>LFIEWL[4x]

Here, we identify an evolutionarily conserved hexapeptide sequence as the major aggregation-prone region (APR) of gastrointestinal peptides of the glucagon family: xFxxWL. We determine nine polymorphic crystal structures of the APR segments of glucagon-like peptides 1 and 2, and exendin and its derivatives. We propose that the pH-dependent changes of the protonation states of glutamate/aspartate residues of APRs initiate switching between the amyloid and the folded, monomeric forms of the hormones. Our results highlight the dual role of short aggregation core motifs in reversible amyloid formation and receptor binding.

Two polymorphic crystal forms could be grown from solutions of APRex-4. In polymorph B of the same system, shifted interfaces could be found which are stabilized by different interactions. A lateral shift between adjacent β-sheets allows the formation of 3 different interfaces (S1, S2, and S3). S3 is stabilized by the hydrophobic interactions of the Leu, Phe, and Ile side chains, plus the intersheet Glu–Glu side chain H-bonds. An aromatic cluster is formed in both polymorphs of APRex-4. At pHs where Glu/Asp side chains become protonated, charge frustration ceases as side chains establish intersheet H-bonds. For example, protonated Glu forms H-bond either with the opposing Glu (S1 of polymorph A, S3 of Polymorph B in APRex-4 Fig. 6c), or with the indole rings of Trp(s) (S2 of Polymorph B Fig. 4e). Polymorphs formed in pure aqueous solution are laterally displaced, as the side chains of Tyr, Glu, and Gln rather form H-bonds with the surrounding water molecules. Aromatic side chains form intrasheet aromatic ladders in the two parallel structures of APRGLP2 and APRTc5b (polymorph D), as well as in both polymorphic structures of APRex-4. Interestingly, exendin-derived hexapeptides showed the greatest structural plasticity that is reflected in multiple β-sheeted conformers giving rise to several polymorphs.> MGIVFTNHNIDLLSVEFDEITKNCNYTFSVDGETAIFTARISIIRNIKGIKYSEELDKFIMSIMPLQPKVSKILGGVTWDCICGKE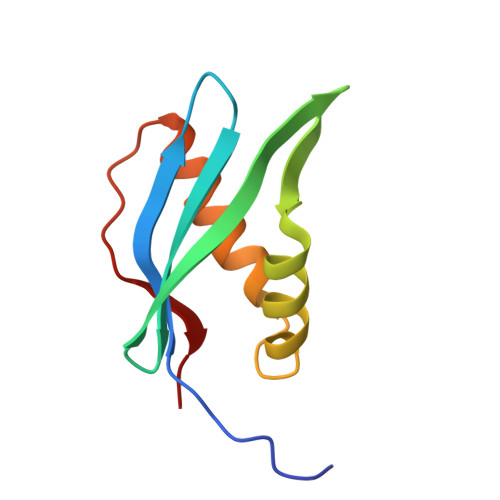VGFPVRLIGK>[2x]ERAGPVTWVMMIACVVVFIAMQILGDQE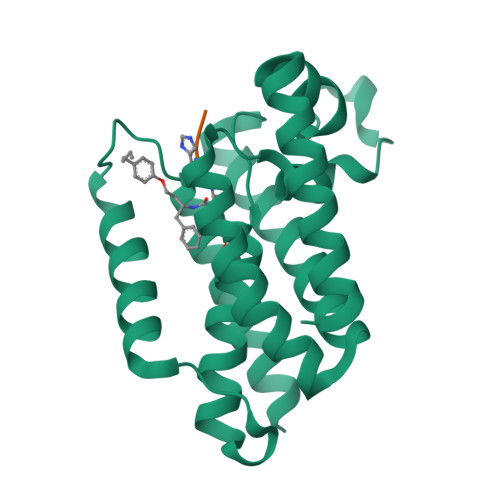VMLWLAWPFDPTLKFEFWRYFTHALMHFSLMHILFNLLWWWYLGGAVEKRLGSGKLIVITLISALLSGYVQQKFSGPWFGGLSGVVYALMGYVWLRGERDPQSGIYLQRGLIIFALIWIVAGWFDLFGMSMANGAHIAGLAVGLAMAFVDSL> MEKTYNLNDILLSNEYEKIKEDIKEEIINDMASKKVKYSNTSEFAKNDFLKDEFIDLVVDGETYEITYGNLI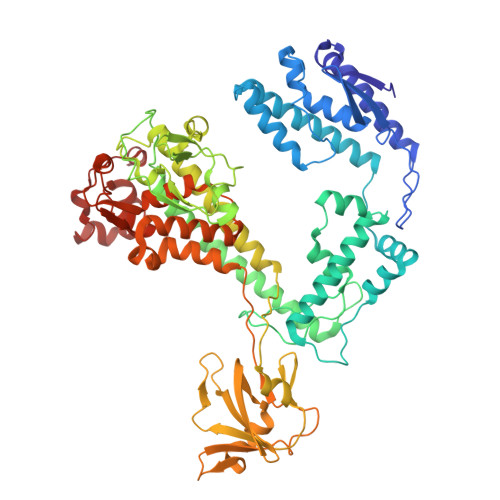TLLIVARPFNHFKVPMTEDLLFDLSDLKEYQNYYTTLLEHFGYSNEIKSIIKDVISELAIFSGDINVTFGNTVSIKSLIDLGNKVKRFRELLHYRLPNDEALEFNDIEAIIKKNLDEIMKILSETDNMLRYYIDSGAGINSKQFGQVLSLVGSKPDLFGKIIPYPINTSFLRGLDVRSFYINALGARKALITNYQQVRNSGYLTRKISMLLMDTKLIDLDDCGSHENNYLSINVENKDVLKRFSKRSYLNNNGELVEIDINDESLIGQVIKIPSPTTCASNEGVCRKCYGKLFDINKDLNIGMIAVLLLTDPLTQRLLSAKHLLETRSSKIDWGTNFEENFIVNRNLIYPKVYNGTVIIKEDDFKEDEETEEQVFDTFTLKSGNRFISISSPMRLFLNKDLKKQLDESFYNIEEMQFEIPLNKLDEGDSFATFIMDNNELSKPLREIKDLIETNKYIKDHNVNEVVNYFIYLLNESGINIQSVHSELIIREMMKLDDSDRTQFKNDKMPDYEIFRITDANLKGDSLSRSLLFEQVKKQLTTLDYDTFNKTKSSILDKLL>[3x]MHHHHHHMPLEPHFMPDFLGHAENPLREEEWARLNETVIQVARRSLVGRRILDIYGPLGAGVQTVPYDEFQGVSPGAVDIVGEQETAMVFTDARKFKTIPIIYKDFLLH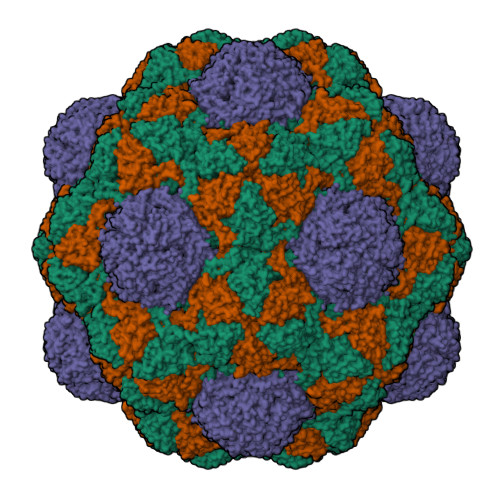WRDIEAARTHNMPLDVSAAAGAAALCAQQEDELIFYGDARLGYEGLMTANGRLTVPLGDWTSPGGGFQAIVEATRKLNEQGHFGPYAVVLSPRLYSQLHRIYEKTGVLEIETIRQLASDGVYQSNRLRGESGVVVSTGRENMDLAVSMDMVAAYLGASRMNHPFRVLEALLLRIKHPDAICTLEGAGATERR> MENTENSVDSKSIKNLEPKIIHGSESMDSGISLDNSYKMDYPEMGLCIIINNKNFHKSTGMTSRSGTDVDAANLRETFRNLKYEVRNKNDLTREEIVELMRDVSKEDHSKRSSFVCVLLSHGEEGIIFGTNGPVDLKKITN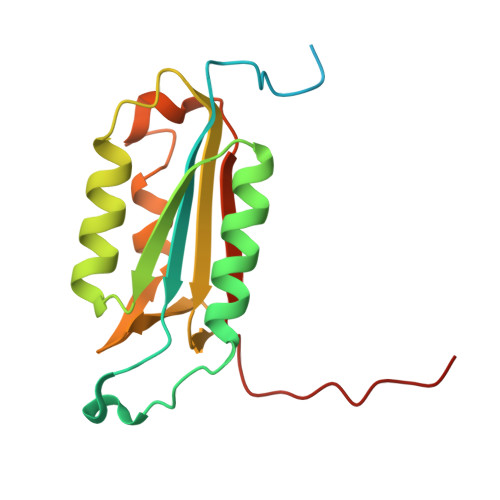FFRGDRCRALTGKPKLFIIQACRGTELDCGIETD N-{2'-[(4-FLUOROPHENYL)AMINO]-4,4'-BIPYRIDIN-2-YL}-4-METHOXYCYCLOHEXANECARBOXAMIDE | C24 H25 F N4 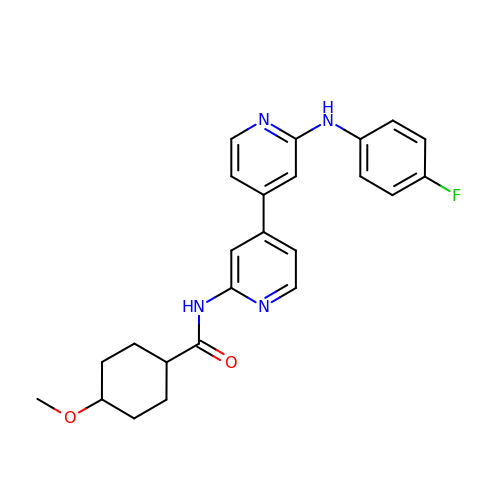O2 | ACGBFWCBVIXTPZ-OQIWPSSASA-N>MFRSRPNALSQRSVIASSSELASLAGRDILKRGGNIFDAALAVSAMLCVTQNNLCGLGGDLFALIRDENGQIMDLNGSGQASRAVSIDYYESMGLTKIPERGPYAAITVPGIAGSWDEIFRKFATMDIADILEPAIRTASAGFPITQNYSDSIARSAPVIGQYRGWSSIFMPNGSVPVAGEILKQPDLAESFRLMSEEGFRSFYDGSLADIIIAGLEGTGSPLSDRDLRVYRPLIGKPVFTDLDEFRIYETSPNSQGITVIEWIRGMESHGYDSRTMWEAKIEDIFETMEEAYDKRRKITDPSYMNIAQHDSANGKKDGLPKRDHNDIGDTTYFSISDSEGRSVSIIQSNYMGFGSGIVPKGTGFVLQNRGSYFTLQRDHPNALMPGKRTFHTLAACMVEKEHDLYASLGSMGGDIQPQVQMQILMEILK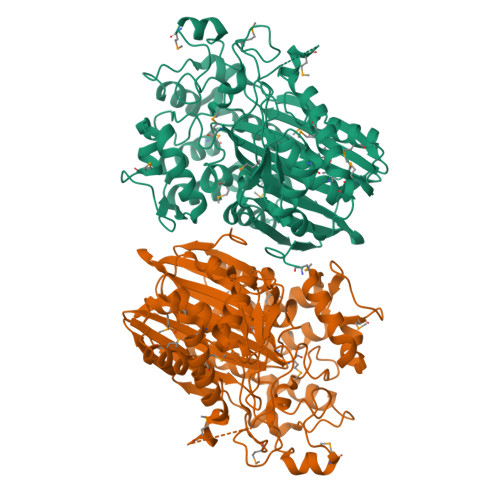DNTDPQAILDKPRWTEPYTIYEAPGAVYVESEELYRNVSKQISGRKVVLRDVSQEFGTAQITTLIRGDVVVGAADPRGDGIAIPYS[4x]1S,3AS,8AS-TRIMETHYL-1-OXIDO-1,2,3,3A,8,8A-HEXAHYDROPYRROLO[2,3-B]INDOL-5-YL 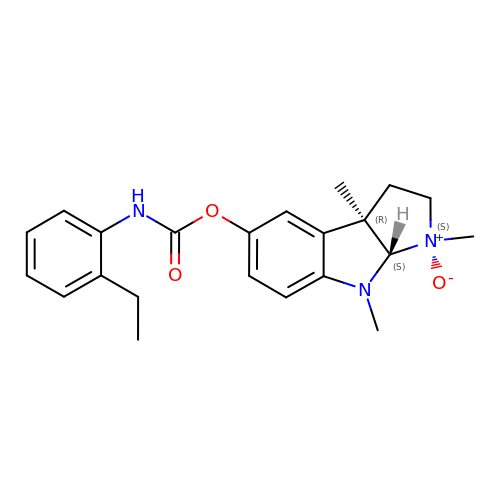2-ETHYLPHENYLCARBAMATE | C22 H27 N3 O3 | MVHRCJQCKYPDRL-UHFFFAOYSA-N> VEPSGHAADRIARLPGQPAVDFDMYSGYITVDEGAGRSLFYLLQEAPEDAQPAPLVLWLNGGPGCSSVAYGASEELGAFRVKPAGAGLVLNEYRWNKVANVLFLDSPAGVGFSYTNTSSDIYTSGDNRTAHDSYAFLAKWFERFPHYKYRDFYIAGESYAGHYVPELSQLVHRSKNPVINLKGFMVGNGLIDDYHDYVGTFE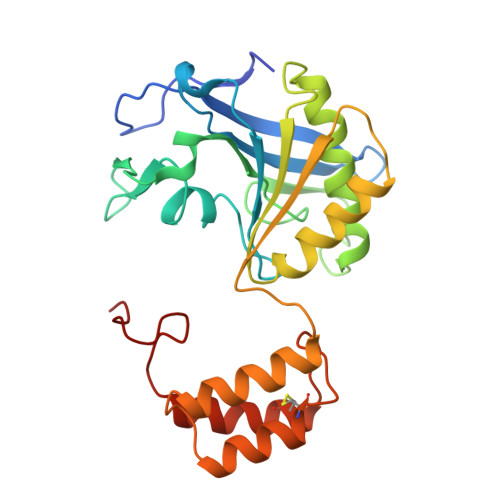FWWNHGIVSDDTYRRLKEACLHDSFIHPSPACDAATDVATAEQGNIDMYSLYTPVCN> MTADELVFFVNGKKVVEKNADPETTLLAYLRRKLGLRGTKLGCGEGGCGACTVMLSKYDRLQDKIIHFSANACLAPICTLHHVAVTTVEGIGSTKTRLH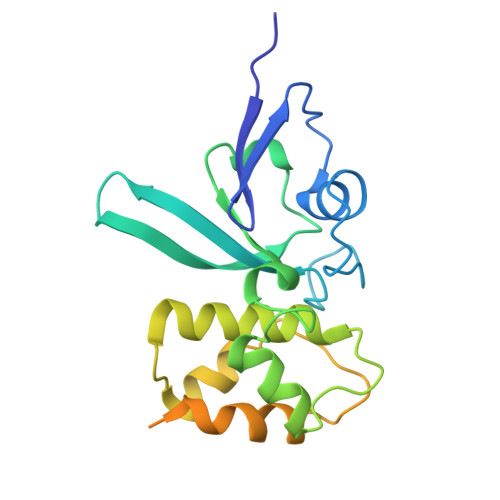PVQERIAKSHGSQCGFCTPGIVMSMYTLLRNQPEPTVEEIEDAFQGNLCRCTGYRPILQGFRTFAKNGGCCGGNGNNPNCCMNQKKDHTVTLSPSLFNPEEFMPLDPTQEPIFPPELLRL> GAAAAMSICPHIQQVFQNEKSKDGVLKTCNAARYILNHSVPKEKFLNTMKCGTCHEINSGATFMCLQCGFCGCWNHSHFLSHSKQIGHIFGINSNNGLLFCFKCEDYIGNIDLINDAILAKYWDDVCTKTMVPSMERRDGLSGLINMGNTCFMSSILQCLIHNPYFIRHSMSQIHSNNCKVRSPDKCFSCALDKIVHELYGALNTKQASSSSTSTNRQTGFIYLLTCAWKINQNLAGYSQQ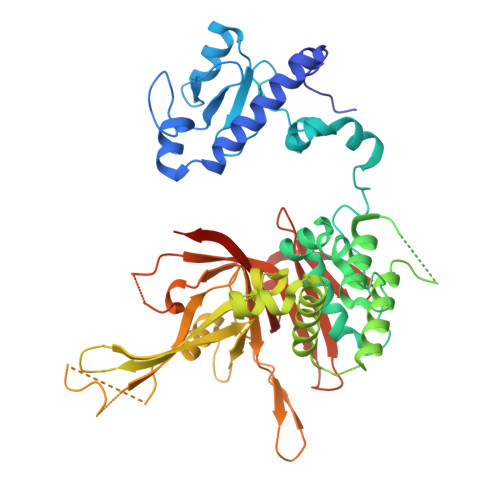DAHEFWQFIINQIHQSYVLDLPNAKEVSRANNKQCECIVHTVFEGSLESSIVCPGCQNNSKTTIDPFLDLSLDIKDKKKLYECLDSFHKKEQLKDFNYHCGECNSTQDAIKQLGIHKLPSVLVLQLKRFEHLLNGSNRKLDDFIEFPTYLNMKNYCSTKEKDKHSENGKVPDIIYELIGIVSHKGTVNEGHYIAFCKISGGQWFKFNDSMVSSISQEEVLKEQAYLLFYTIRQVN4-(5-PYRIDIN-4-YL-1H-1,2,4-TRIAZOL-3-YL)PYRIDINE-2-CARBONITRILE 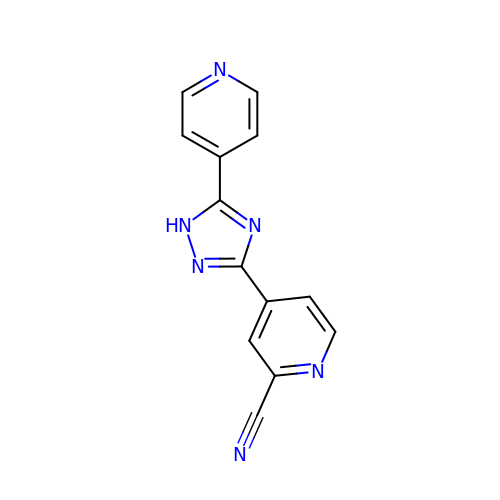| C13 H8 N6 | UBVZQGOVTLIHLH-UHFFFAOYSA-N>MHHHHHHSSGTDDDDKAMATTATEAAKAAPAEQANGNANGEQKTRHSEVGHKSLLKSDDLYQYILDTSVYPREPESMKELREITAKHPWNLMTTSADEGQFLNMLIKLIGAKKTMEIGVYTGYSLLATALALPEDGTILAMDINRENYELGLPCIEKAGVAHKIDFREGPALPVLDDLIADEKNHGSFDFVFVDADKD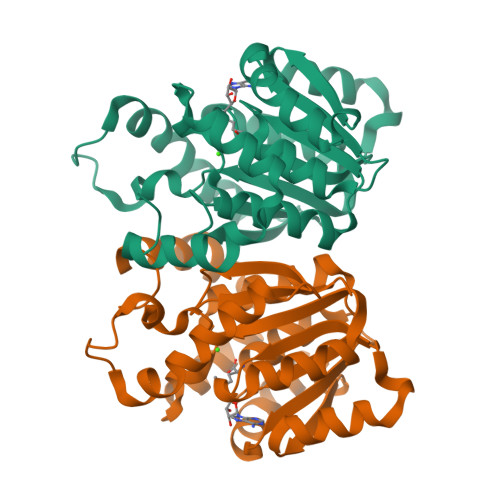NYLNYHDRLLKLVKLGGLIGYDNTLWNGSVVLPDDAPMRKYIRFYRDFVLVLNKALAADERVEICQLPVGDGVTLCRRVK[2x]> SMQELQGLDYCKPTRLDLLLDMPPVSYDVQLLHSWNNNDRSLNVFVKEDDKLIFHRHPVAQSTDAIRGKVGYTRGLHVWQITWAMRQRGTHAVVGVATADAPLHSVGYTTLVGNNHESWGWDLGRNRLYHDGKNQPSKTYPAFLEPDETFIVPDSFLVALDMDDGTLSFIVDGQYMGVAFRGLKGKKLYPVVSAVWGHCEIRMRYLNGLDPE;> NELNNNLPGGAPAAP

The SPRY domain- and SOCS box-containing proteins, SPSB1 to SPSB4 (also known as SSB-1 to -4), contain a protein interaction domain known as the SPRY domain, which was first identified as a sequence repeat in the dual-specificity kinase splA and ryanodine receptors, together with a C-terminal SOCS box motif. The presence of the SOCS box motif suggests that the SPSB proteins may function as part of an E3 ubiquitin ligase, with the SPRY domain determining the substrate(s) for ubiquitination, and this has been confirmed recently for SPSB2 (Z.K., R.S.L., R.S.N., and S.E.N., personal communication). All three hSPSB proteins share the same conserved SPRY domain fold with two short N-terminal helices packed against a bent β-sandwich, comprising two 7-stranded β-sheets. The structures show remarkable conservation of the SPRY domain fold and absolute sequence conservation for positions in contact with the (E/D)(L/I)NNN motif.

The structure of hSPSB1 bound to hPar-4(67–81) was refined to 1.79 Å resolution, enabling direct comparison of the hPar-4 and VASA binding modes in hSPSB1. Residues Asn67-Pro74 from hPar-4 were well defined, corresponding to the minimal binding motif determined by NMR chemical shift changes. Further electron density was not present to build the C-terminal residues (75–81, GGAPAAP), suggesting that, as for VASA, the N-terminal site is sufficient for high-affinity interaction. The hPar-4 and VASA peptides adopt similar conformations, with tight superimposition of the conserved NNN motifs, which form a total of six conserved hydrogen bonds, including two between hPar-4 Asn70 and hSPSB1 Thr111 (side and main chain), one between Asn71 and the Gly218 carbonyl, and three from Asn72 to Arg77, Tyr129, and the Val216 carbonyl. One further conserved main chain–main chain hydrogen bond is formed between Asn70 of hPar-4 and the Gly218 amide of hSPSB1. Towards the N-terminus, the Glu68 carboxyl moiety of hPar-4 overlays well with VASA Asp184 to hydrogen bond with hSPSB1 Tyr129 (equivalent to SPSB2 Tyr120) and the three main-chain amides of the NNN motif. However, the longer Glu68 side chain of hPar-4 reorients the backbone to replace this bond with the somewhat unfavorable 3.3-Å juxtaposition of the Glu68 β-carbon with the hPar-4 Asn72 carbonyl. At the N-terminus, the hPar-4 residue Asn67 makes no contact with hSPSB1. To the C-terminus of the NNN motif, the introduction of a proline residue (Pro74) also induces a main-chain shift; in VASA, the preceding residue, Asn189, makes both main-chain amide and carbonyl hydrogen bonds to the hSPSB1 backbone, but in hPar-4, only the amide bond can form. Neither Leu73 nor Pro74 in hPar-4 makes a significant contribution to binding.>MRGSHHHHHHGLVPRGSMIRTMLQGKLHRVKVTHADLHYEG[2x];>[2x]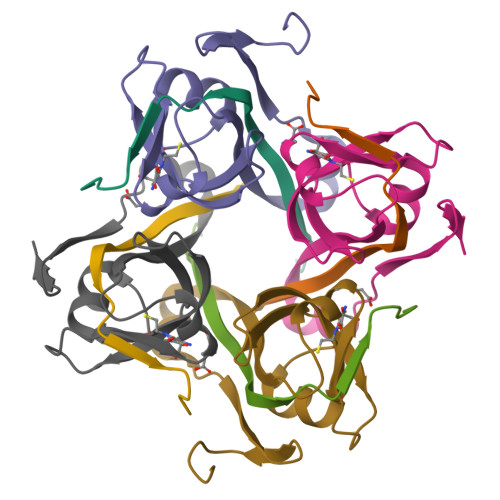XCAIDQDFLDAAGILENEAIDIWNVTNGKRFSTYAIAAERGSRIISVNGAAAHCASVGDIVIIASFVTMPDEEARTWRPNVAYFEGDNEMKRTAKAIPVQVA(betaS)-Nalpha-{4-[4-(4-aminophenyl)buta-1,3-diyn-1-yl]benzoyl}-N,beta-dihydroxy-beta-methyl-L-tyrosinamide 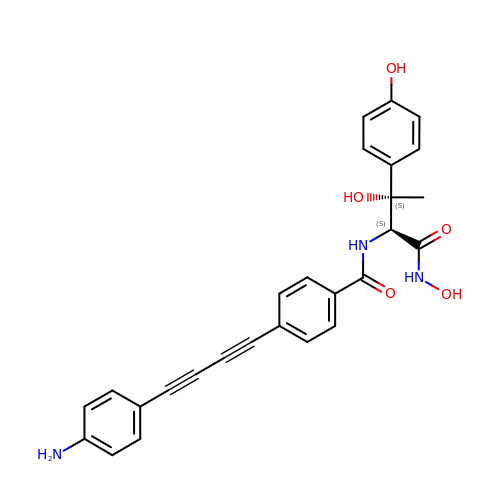| C27 H23 N3 O5 | CXPNZJDYPDDMKA-SQHAQQRYSA-N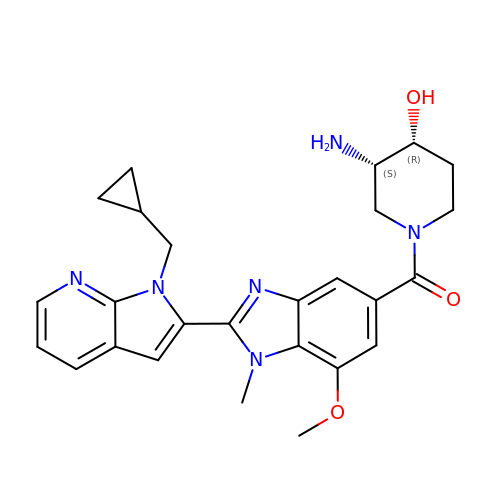[(3S,4R)-3-amino-4-hydroxypiperidin-1-yl]{2-[1-(cyclopropylmethyl)-1H-pyrrolo[2,3-b]pyridin-2-yl]-7-methoxy-1-methyl-1H-benzimidazol-5-yl}methanone | C26 H30 N6 O3 | SHBUAYSOPVZNDD-GHTZIAJQSA-N(1S)-1,5-anhydro-1-(4-chloro-2,5-dihydroxyphenyl)-D-glucitol 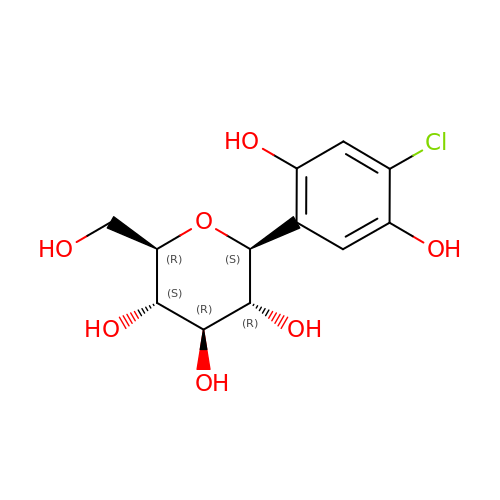| C12 H15 Cl O7 | LHMIFDKRIZSEFV-ZIQFBCGOSA-N>[3x]GPKVPEFGSSRISALEYATTRKKSEVVYSGVSVTIPTAPTNLVSLLKTLTPSSGTLAPFFDTVNNKMVVFNENKTLFFKLSIVGTWPSGTANRSMQLTFSGSVPDTLVSSRNSATTTDNILLATFFSVDKDGFLATNGSTLTIQSNGAAFTATTIKIIAEQ

The six trimeric tailspikes (above) are bound to the lower sides of the tail, and a single trimer of the product of P22 gene 26 (gp26) forms a long “needle” that extends outward from the center of the base of the tail. The N-terminal, virion-proximal end of the gp26 needle forms the exit channel plug that traps packaged DNA in the virion. The long shaft domains have a three-strand coiled-coil structure with 11–16 repeats of heptad amino acid sequences, and the N-terminal 27 residues fold back on the surface of the coiled-coil in the P22 structure to form what may be the site through which the needle binds in the tail channel to form the plug. We report here the X-ray structure of the C-terminal domain of the phage HS1 needle (HS1 is an E. coli P22-like phage with an Sf6-like needle) which confirms the very unusual feature that this protein domain binds three L-glutamate molecules.

The HS1 tail needle (encoded by locus_tag EcHS_A0316 gene) is characterized by a virion-binding N-terminal domain 98% identical to that of Sf6, and a shaft-forming coiled-coil helical region predicted to be 210 Å long that is only 67% identical in sequence to Sf6. The C-terminus of the HS1 tail needle contains a domain (the knob) that is 99% identical to Sf6 in sequence. We cloned the HS1 prophage needle’s C-terminal knob and nine residues of its coiled-coil helical shaft fused to maltose binding protein (MBP) after polymerase chain reaction (PCR) amplification from E. coli strain HS DNA. The globular HS1 needle knob folds into a homotrimeric TNF-like fold, very similar to that of the Sf6 knob (rmsd 0.137 Å). The trimer is built with three identical subunits each displaying a jellyroll topology characterized by seven stacked anti-parallel ß-strands. Like the Sf6 knob, the HS1 tail knob structure contains a phosphate ion bound at the distal tip of the knob and an L-glutamate is present in the electron density at each of the three dimeric interfaces of the homotrimer. The phosphate ion makes polar contacts with HS1 needle residues S266 and N268 near the 3-fold axis at the distal tip of the knob. Alteration of these residues in Sf6 knob did not affect the stability of the protein. The conserved triad, S266-R267-N268, is present in all the known needle knob sequences from P22-like phages; however, although R267 (its side chain points down and is involved in intra-chain stability) is universally present in all the proteins aligned in figure S3, the S and N on either side are not conserved in proteins encoded by the non-P22-like phages, so the bound phosphate is unlikely to be a universal feature of all of these proteins. Although not surprising given the similarity of the two proteins, the presence of the bound glutamate molecules in the HS1 structure is consistent with their being universally present in the P22-like needle knob structures.The only de novo biosynthetic pathway to generate dTTP (2′-deoxythymidine-5′-triphosphate) requires reductive methylation of dUMP (2′-deoxyuridine-5′-monophosphate) to dTMP (2′-deoxythymidine-5′-monophosphate) by TS. The TS enzyme is an obligatory homodimer whose subunits associate with nanomolar affinity to form a dimer that adopts an asymmetric conformation upon substrate binding. Inhibition of TS leads to the cessation of DNA replication and thymineless death of proliferating cells, which renders the enzyme an attractive target for cancer chemotherapy. Ligand-free TS protein binds its own mRNA and thereby represses translation.

To gain direct insight into the molecular recognition of mRNA by hTS, we attempted co-crystallization of the enzyme with oligonucleotide constructs representing the TS site 1 motif. X-ray data sets were collected and structures determined for crystals grown at low salt (100 mM buffer) as well as high salt (1.75 M ammonium sulphate) concentration. Molecular replacement with previously published hTS coordinates furnished structures with the enzyme adopting either of the previously observed active and inactive conformations of the loop regions about I108-G129 and A181-A197; however, each without RNA bound. In the active conformation, the catalytic C195 is located in the active site, while it resides at the dimer interface in the inactive conformation. Crystallization of hTS at low salt may have led to discrimination against RNA ligand binding by crystal contacts that involve the putative RNA-binding region. Although the crystallography effort furnished structures of the protein in both the active and inactive conformation, co-crystallization of an hTS–RNA complex remained elusive.

>[4x]MPVAGSELPRRPLPPAAQERDAEPRPPHGELQYLGQIQHILRCGVRKDDRTGTGTLSVFGMQARYSLRDEFPLLTTKRVFWKGVLEELLWFIKGSTNAKELSSKGVKIWDANGSRDFLDSLGFSTREEGDLGPVYGFQWRHFGAEYRDMESDYSGQGVDQLQRVIDTIKTNPDDRRIIMCAWNPRDLPLMALPPCHALCQFYVVNSELSCQLYQRSGDMGLGVPFNIASYALLTYMIAHITGLKPGDFIHTLGDAHIYLNHIEPLKIQLQREPRPFPKLRILRKVEKIDDFKAEDFQIEGYNPHPTIKMEMAVHHHHH>[2x]MNLPTAQEVQGLMARFIELVDVGDIEAIVQMYADDATVESPFGQPPIHGREQIAAHYRQWLGGGKFRVSLTGPVRASHNGSGAMPLRKEWVWN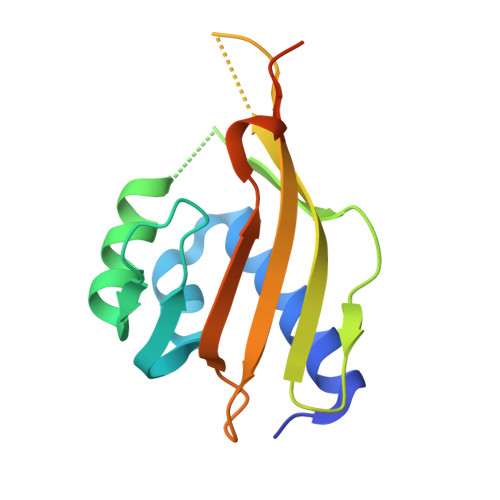GQPSALDVILVMRFDEHGRIQTEQRYWSEVNLSVREPQGSLEHHHHHH>GHHHHHHELNGPLVLVSNNQNIHFNLSLENFLLNNYNDLLKYLNINTIEKFNEPILFLWRNNRSIIIGKNQNIWSECNLKNIKEDGVLVARRFTGGGAVYHDLGNVCFTFLNNNINTSSNFLIILNTLKNHFNIEAKTQGRNDITVNDQKCSGSAFKKIKDVFLHHGTILINLEKNILNKYLTPDKIKYIKHGVSSVNARTINLSEINNNITCENLCIALIKEFTKFYEQNYNTNIIPNDITVHYIDQNNNITKNPEFLKYYN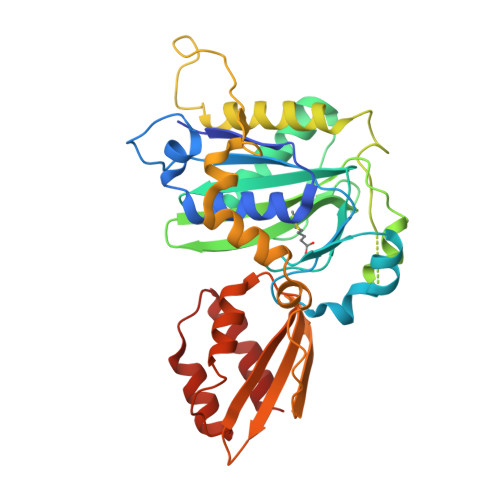LLKDWDWCYGKTPKFQNHIWKQFTFGKLELFFNVSNGFIKDGNIFSDCLDINLIDHLKSIFNNDIKYSKEDISIFFKKLNVENKNYLDEVRSWILQE[2x]>EAEEDGDLQCLCVKTTSQVRPRHITSLEVIKAGPHCPTAQLIATLKNGSKICLDLQAPLYKKIIKKLLES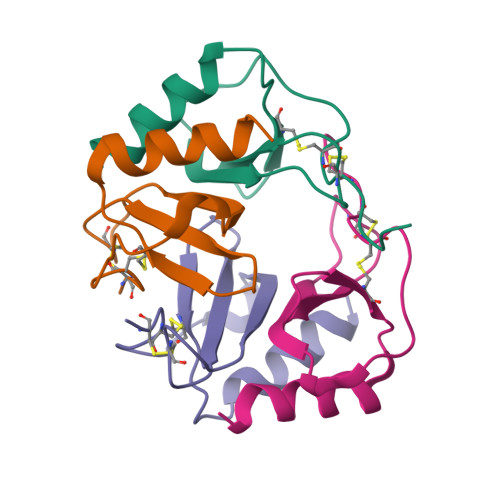[4x]>RHMKVLLLGFEFLPVKVGGLAEALTAISEALASLGHEVLVFTPSHGRFQGEEIGKIRVFGEEVQVKVSYEERGNLRIYRIGGGLLDSEDVYGPGWDGLIRKAVTFGRASVLLLNDLLREEPLPDVVHFHDWHTVFAGALIKKYFKIPAVFTIHRLNKSKLPAFYFHEAGLSELAPYPDIDPEHTGGYIADIVTTVSRGYLIDEWGFFRNFEGKITYVFNGIDCSFWNESYLTGSRDERKKSLLSKFGMDEGVTFMFIGRFDRGQKGVDVLLKAIEILSSKKEFQEMRFIIIGKGDPELEGWARSLEEKHGNVKVITEMLSREFVRELYGSVDFVIIPSYFEPFGLVALEAMCLGAIPIASAVGGLRDIITNETGILVKAGDPGELANAILKALELSRSDLSKFRENCKKRAMSFSWE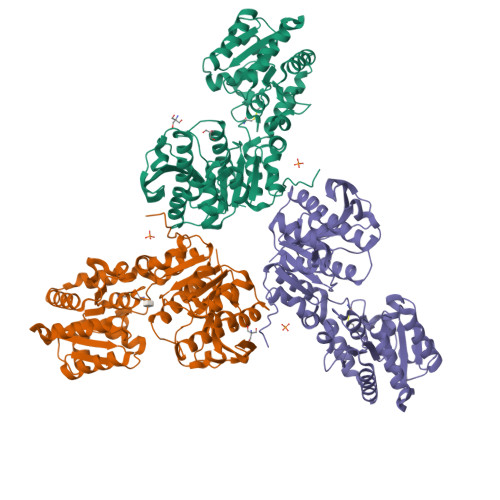KSAERYVKAYTGSIDRAFDFIL[3x]> MIKNECEKDNQLAARLAKLAGYEKVNGFYKFVNTPEKEMENLGGLLKIVKNLFPDSEEQLLSEYFLELDPNKKCARQSVEYSDINQWDTLTDKIIINLCNSKNSTSQEWGKVYSLHRKLNKNEISLNDAIRESGKCKIKSAEMLFFSNAMLMYAYLNIGEFGLMKSTSKLLEFDDLPEGFIKESFKSRVSMLEANISLNENSLLEARQHSNRAIENSNVNRICFFAYLTIGNTLIFEDYDEAKKAY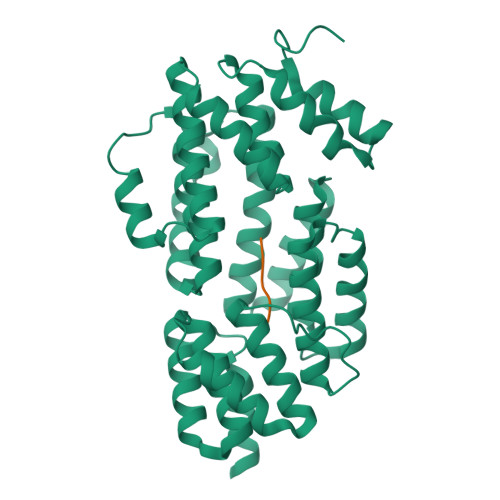IKGQKYAKNPVHQEMLDGALCFLSNIWKKENQWVNYNSDNIKYLQLRAFYYINQGNIEEATEILDELSSRDQDENELGFYYYYKGLISQDKTDYAKSIRYFKKSDDKYFIQLPLLQLERMGADLELLNLISI;> SAIRGA> MGPHHHHHHLESTSLYKKAGSAMEATPTPADLFSEDYLVDTLDGLTVDDQQAVLASLSFSKFLKHAKVRDWCAQAKIQPSMPALRMAYNYFLFSKVGEFIGSEDVCNFFVDRVFGGVRLLDVASVYAACSQMNAHQRHHICCLVERATSSQSLNPVWDALRDGIISSSKFHWAVKQQNTSKKIFSPWPITNNHFVAGPLAFGLRCEEVVKTLLA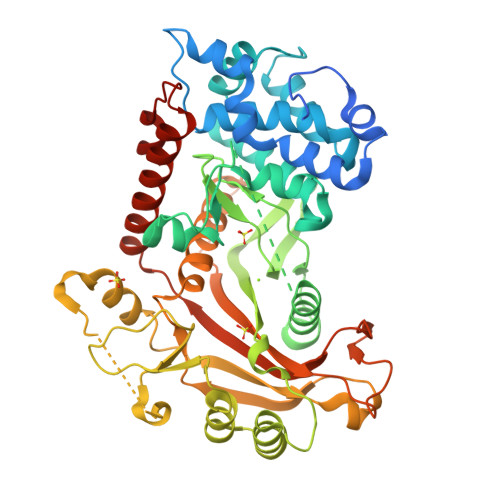TLLHPDETNCLDYGFMQSPQNGIFGVSLDFAANVKTDTEGRLQFDPNCKVYEIKCRFKYTFAKMECDPIYAAYQRLYEAPGKLALKDFFYSISKPAVEYVGLGKLPSESDYLVAYDQEWEACPRKKRKLTPLHNLIRECILHNSTTESDVYVLTDPQDTRGQISIKARFKANLFVNVRHSYFYQVLLQSSIVEEYIGLDSGIPRLGSPKYYIATGFFRKRGYQDPVNCTIGGDALDPHVEIPTLLIVTPVYFPRGAKHRLLHQAANFWSRSAKDTFPYIKWDFSYLSANVPHSP>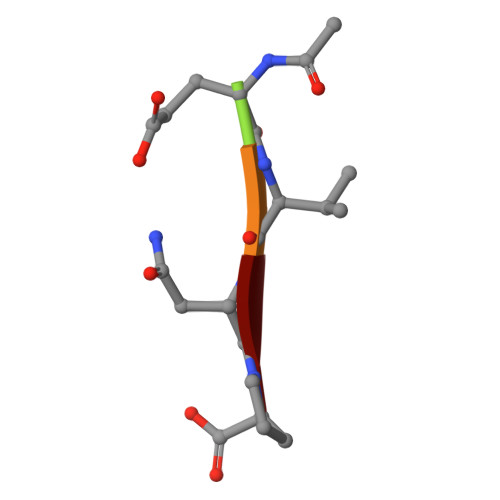 XEVNP>GPLLLKDRKGRAYLVFPKEGGVFHHHKGSVPHEALLE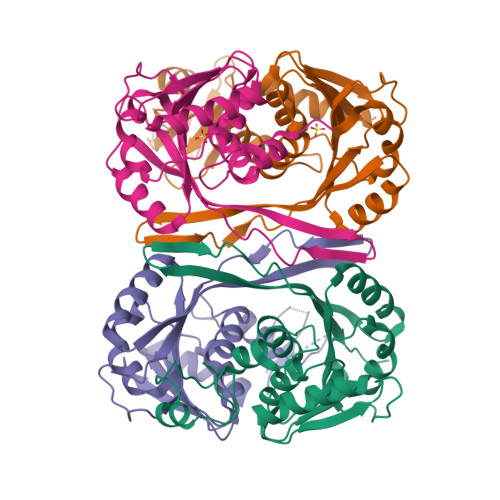AGPGGVVRTHLGEELSVHRPTLEEYLLHMKRSATPTYPKDASAMVTLLDLAPGMRVLEAGTGSGGLTLFLARAVGEKGLVESYEARPHHLAQAERNVRAFWQVENVRFHLGKLEEAELEEAAYDGVALALMEPWKVLEKAALALKPDRFLVAYLPNITQVLELVRAAEAHPFRLERVLEVGWREWEVRLPVAHPRFQQVGHTAFLVALRRWKGS[4x]> MKDNTVPLKLIALLANGEFHSGEQLGETLGMSRAAINKHIQTLRDWGVDVFTVPGKGYSLPEPIQLLNAKQILGQLDGGSVAVLPVIDSTNQYLLDRIGELKSGDACIAEYQQAGRGRRGRKWFSPFGANLYLSMFWRLEQGPAAAIGLSLVIGIVMAEVLRKLGADKVRVKWPNDLYLQDRKLAGILVELTGKTGDAAQIVIGAGINMAMRRVEESVVNQGWITLQEAGINLDRNTLAAMLIRELRAALELFEQEGLAPYLSRWEKLDNFINRPVKLIIGDKEIFGISRGIDKQGALL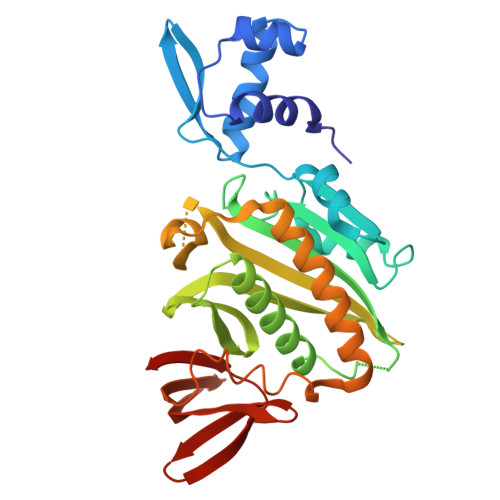LEQDGIIKPWMGGEISLRSAEK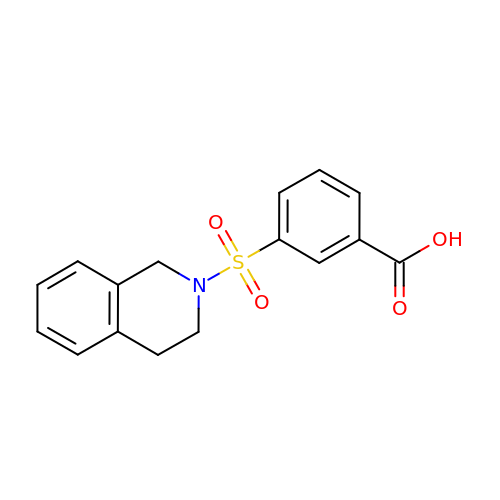3-(3,4-dihydroisoquinolin-2(1H)-ylsulfonyl)benzoic acid | C16 H15 N O4 S | ZGVIUMKHTXKKOX-UHFFFAOYSA-N>[4x]MKIKRIEVLINNGSVPGIPMILNEIQDAIKTVSWPEGNNSFVINPVRKGNGVKPIKNSCMRHLHQKGWALEHPVRIKAEMRPGPLDAVKMIGGKAFAL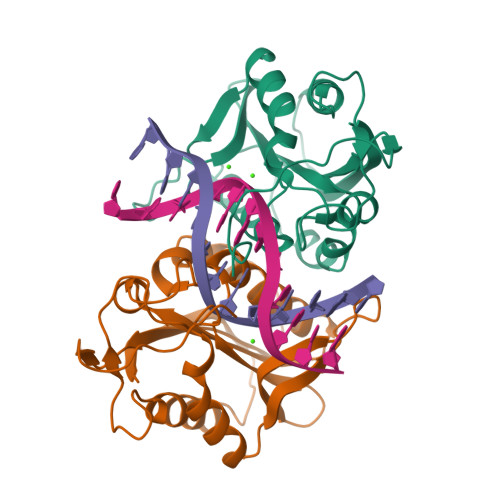EWETGNISSSHRAINKMVMGMLERVIIGGVLILPSRDMYNYLTDRVGNFRELEPYFSVWRQFNLKDAYLAIVEIEHDSVDAQVSLIPKGTDGRAIR> MAAKTIPFVASTALGERLFAGVQKVLAAAKAPVSLVQTDAKFAPADAKYLLAEPLSAAATGELANKYGLSSKVTSGAASQFYPNSIYPSLNVEVVQNLYALSNPAFSSLSATTTKAVTVKDESAIKLAELQKETERNISSFFRDEANKSV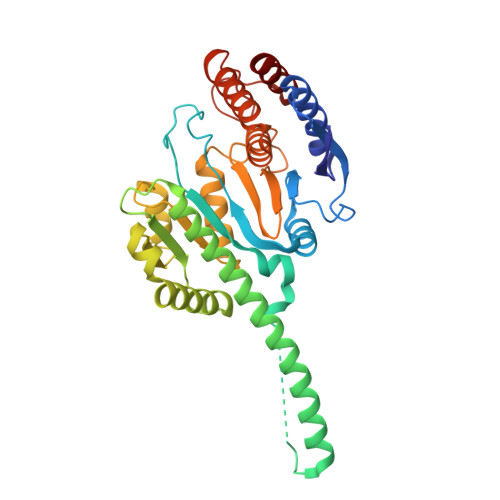QATLRLACDKAIKTKADKKTVMVVTKPHGDAFDDLLAQVTKSESDGRADELRNSSVSVEPTLVGNAWPKLVMFPEGVNVVVCGPNASGDQVAQLFVGIAGGTGMVAQQLVGDAVVFTSANAEDNENPTGALLAASNLLTALGHEAEAKKIAAAVAKAYTTDRILPKELPGGKADLEAFIDAVAKHASA>[3x]DCNTKTATGPYILDRYKPKPVTVSKKLYSATRYTTSAQNELLTAGYRTAWVAYCYNGGLVDSNTGCNARLLHYPPSRDELLLWGSSHQCSYGDICHDCWGSDSYACLGQLDPAKHWAPRKELVRRDANWKFAYHMCNIDWRCGVTTSPVFFNLQWVKNEVKVSTLLPNGSTVEHSAGEPLFWTEKDFSYLVKDNFEIQREEVKISCFVDPDYWVGERKTKKAFCQDG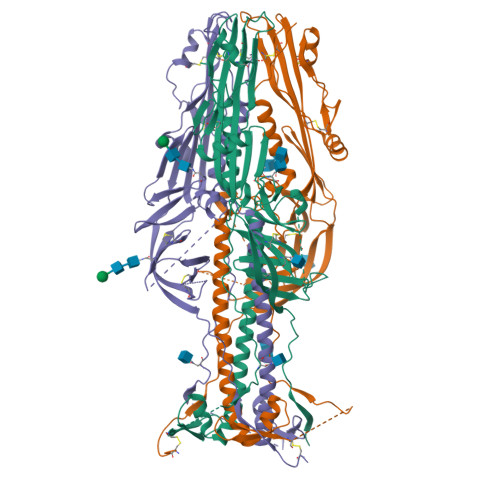TNFFEVTSHQFCHQYACYNFSKDELLEAVYKERAHEKSKDLPFGNKSWTVVTASIDDLHALSAAQAFELEGLRASFAELDSRFRQLSEILDTVISSIAKIDERLIGRLIKAPVSSRFISEDKFLLHQCVDSVANNTNCVGDSAYVDGRWTHVGDNHPCTTVVDEPIGIDIYNFSALWYPSAAEVDFRGTVQSEDGWSFVVKSKDALIQTMMYTKNGGKGTSLTDLLDYPSGWLKGQLGG> GPSQVIFNSVEKFYIPGGDVTCHYTFTQHFIPRRKDWIGIFRVGWKTTREYYTFMWVTLPIDLNNKSAKQ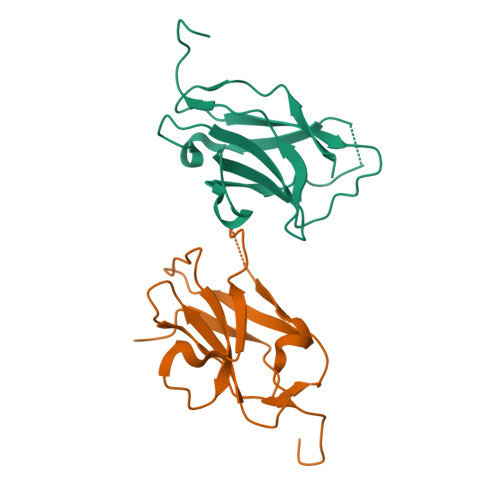QEVQFKAYYLPKDDEYYQFCYVDEDGVVRGASIPFQFRPENEEDILVVTTQGE> DGETCAIPAPFTRRIVGRDGLCVDVRNGYDTDGTPIQLWPCGTQRNQQWTFYNDKTIRSMGKCMTANGLNSGSYIMITDCSTAAEDATKWEVLIDGSIINPSSGLVMTAPSGASRTTLLLENNIHAASQGWTVSNDVQPIATLIVGYNEMCLQANGENNNVWMEDCDVTSVQQQWALFDDRTIRVNNSRGLCVTSNGYVSKDLIVIRKCQ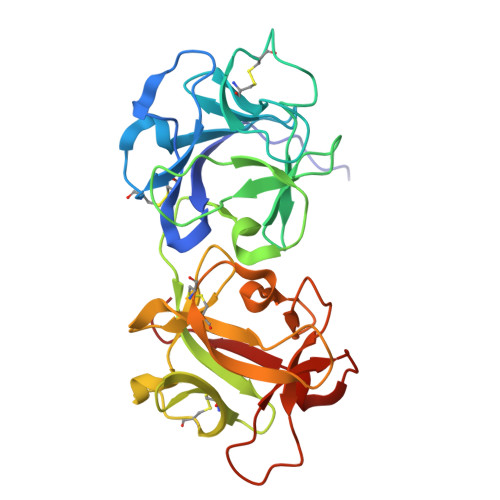GLATQRWFFNSDGSVVNLKSTRVMDVKESDVSLQEVIIFPATGNPNQQWRTQVPQI> SNAVMSGNKGTNYEKLYLGMDFGTSGGRFTVIDEQGEIKAQGKREYPPFMKEESMGWASSWKATLFSLLEDIPVTVRSLVSSISLDGTSATTLILNSESGEVLCQPYLYNQSCPDALPEVKSIAPANHTVCSGTSTLCKLVSWWNTEVPNRESAVLLHQADWLLWLLHGRLGVSDYNNALKVGYDPESESYPSWLLGQPYSQLLPKVQAPGTSIGNLKESFTRQFGFPDDCIVCTGTTDSIAAFLAARATEPGKAVTSLGSTLAIKLLSTKRVDDARYGVYSHRLDDKWLVGGASNTGGAILRQLFSDEQLERLSQEINPMVGSPLDYYPLQSSGERFPIADPNLAPRLLPRPESDV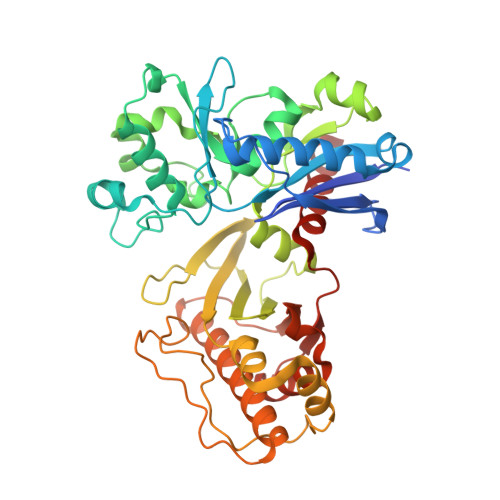EFLHGILESIARIEGKGYKLLKELGATEAEEVLTAGGGAKNDKWIKIRQRVLGLPVKKAVHTEASYGASLLALKGAKQNSGL> ENALL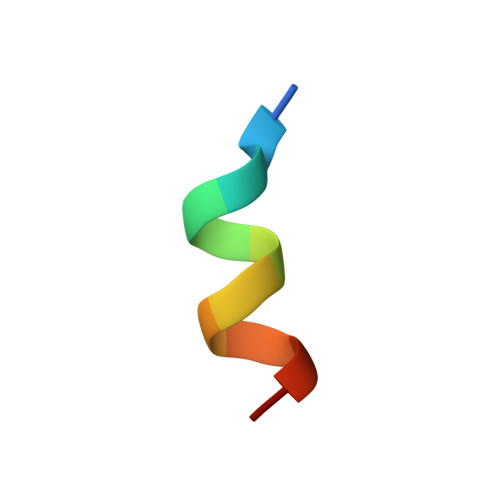RYLLDKD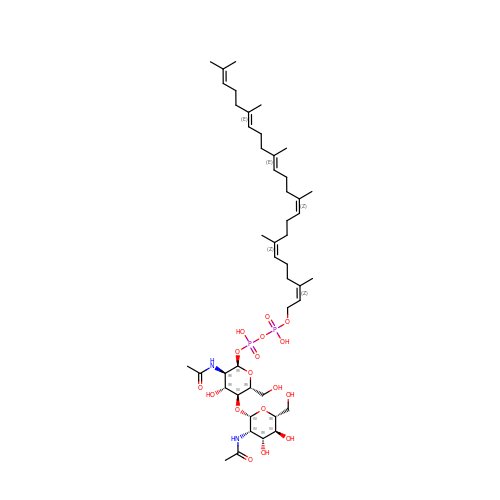2-(acetylamino)-4-O-[2-(acetylamino)-2-deoxy-beta-D-mannopyranosyl]-2-deoxy-1-O-[(S)-{[(R)-{[(2Z,6Z,10Z,14E,18E)-3,7,11,15,19,23-hexamethyltetracosa-2,6,10,14,18,22-hexaen-1-yl]oxy}(hydroxy)phosphoryl]oxy}(hydroxy)phosphoryl]-alpha-D-glucopyranose | C46 H78 N2 O17 P2 | MUXGVGLOWSLCMK-NSGWRCNHSA-N> MKPVTLYD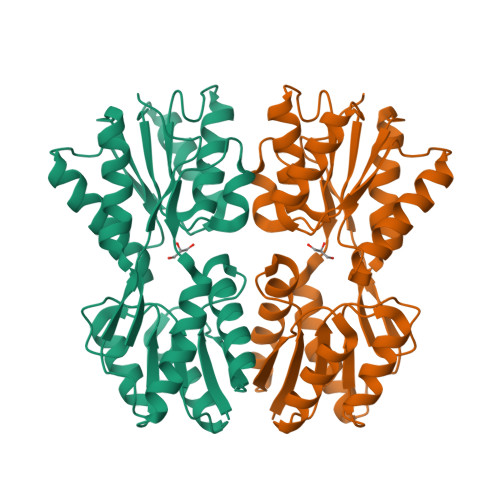VAEYAGVSYQTVSRVVNQASHVSAKTREKVEAAMAELNYIPNRVAQQLAGKQSLLIGVATSSLALHAPSQIVAAILSRADQLGASVVVSMVERSGVEACKTAVHNLLAQRVSGLIINYPLDDQDAIAVEAACTNVPALFLDVSDQTPINSIIFSHEDGTRLGVEHLVALGHQQIALLAGPLSSVSARLRLAGWHKYLTRNQIQPIAEREGDWSAMSGFQQTMQMLNEGIVPTAMLVANDQMALGAMRAITESGLRVGADISVVGYDDTEDSSCYIPPLTTIKQDFRLLGQTSVDRLLQLSQGQAVKGNQLLPVSLVKRKTTLAPNTQTASPRALADSLMQL> ALPDQIDVKVKNLTPEDTIYDRTRQVFYQSNLYKGRIEVYNPKTQSHFNVVIDGASSNGDGEQQMSGLSLLTHDNSKRLFAVMKNAKSFNFADQSSHGASSFHS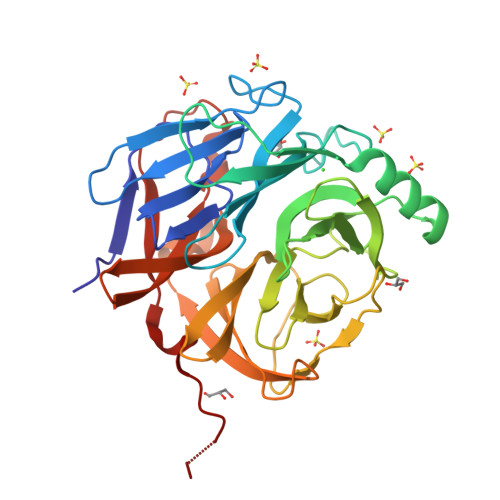FNLPLSENSKPVWSVNFEKVQDEFEKKAGKRPFGVVQSAQDRDGNSYVAFALGMPAIARVSADGKTVSTFAWESGNGGQRPGYSGITFDPHSNKLIAFGGPRALTAFDVSKPYAWPEPVKINGDFGTLSGTEKIVTVPVGNESVLVGARAPYAISFRSWDNWKSANIKKTKRSELQNSGFTAVADYYQGSEQGLYAVSAFFDNGAHGGRSDYPLYKLDNSIQNFHHHHHH> MAKSHHHHHHTSTKAERWQARKDLIAKGSNSLYPDAQIAAKRLAANNIAVEKAKLAENVYKTVNPLEATPGVPEGWKDISNDAGALKKYGLDKEVLFDHADTPDFLARVYQPD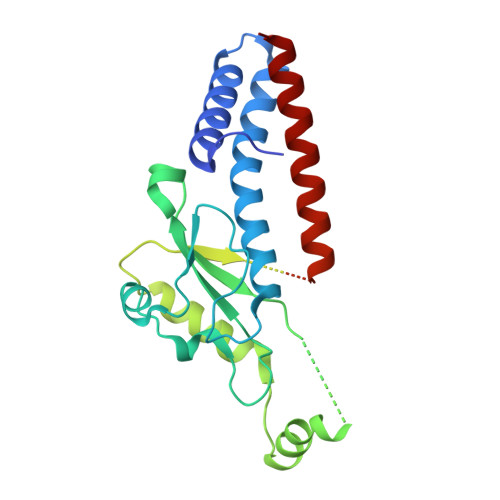SAVFGSDMNPTIVFRGSRQPEFFPTKNMADWINNGAQGLGMESDYYKRAVRLGSRLAKSVSKIDIAGHSLGGGLASATSIASGQAGWTFNAAGLHSTTVEKYGGSLLGEADNIQAYRVEGELLTKIQEVNLAEDYKMLKGHIPTLIAKEEISAIMPNAAGVVHDLPGGTGGPLDRHGIGQAIDCIEQQKDEDISIIRSRA> STQTSRVTLVGEMLPAYNEILTPEALSFLKELHENFNERRIELLQKRMKKQQKIDAGEFPKFLEETKRIREADWTIAKLPKDLEDRRVEITGPVDRKMVINALNSGAHLFMADFEDSNSPTWENAIEGQINLRDAVKGTISHKNENGKEYRLNSKTAVLIVRPRGWHLEEKHMQVDGKNMSGSLVDFGLYFFHNAKALLEKGSGPYFYLPKMESYLEAR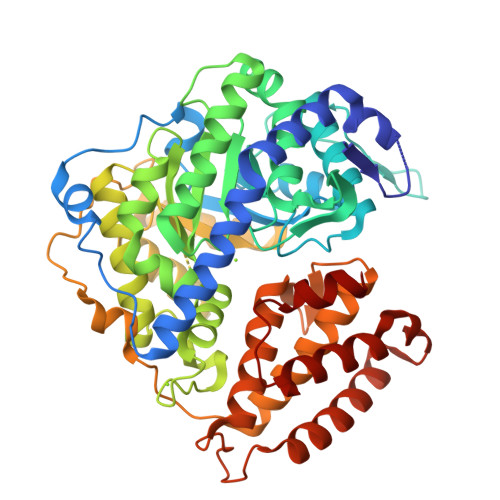LWNDVFVFAQKYIGIPNGTIKATVLLETIHASFEMDEILYELKDHSAGLNCGRWDYIFSFLKAFRNHNEFLLPDRAQVTMTAPFMRAYSLKVIQTCHRRNAPAIGGMAAQIPIKNNPEANEAAFEKVRADKEREALDGHDGTWVAHPGLVPVAMEVFNHIMKTPNQIFRKREEIHVTEKDLLEVPVGTITEEGLRMNISVGIQYIASWLSGRGAAPIYNLMEDAATAEISRAQVWQWIRHEGGKLNDGRNITLELMEELKEEELAKIEREIGKEAFKKGRFQEATTLFTNLVRNDEFVPFLTLPGYEIL4-(1-ethyl-3-pyridin-3-yl-pyrazol-4-yl)-~{N}-(4-piperazin-1-ylphenyl)pyrimidin-2-amine 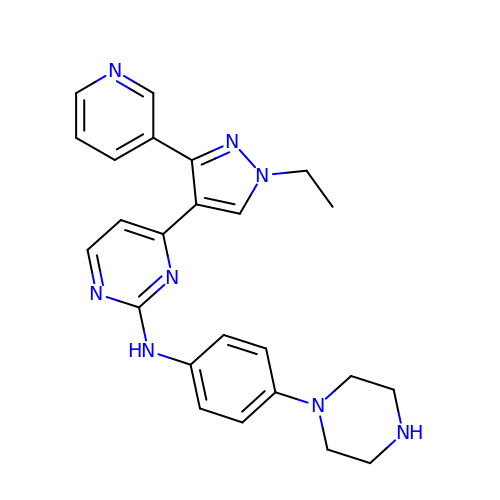| C24 H26 N8 | FOCILHGCJYYBPA-UHFFFAOYSA-N> MALLNIFDIAGSALAAQSKRLNVAASNLANADSVTGPDGQPYRAKQVVFQVDAAPGQATGGVKVASVIESQAPEKLVYEPGNPLADANGYVKMPNVDVVGEMVNTMSASRSYQANIEVLNTVKSMM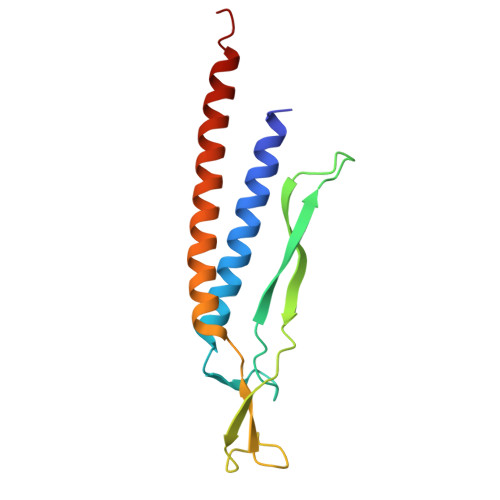LKTLTLGQ>AQCSVDIQGNDQMQFNTNAITVDKSCKQFTVNLSHPGNLPKNVMGHDWVLSTAADMQGV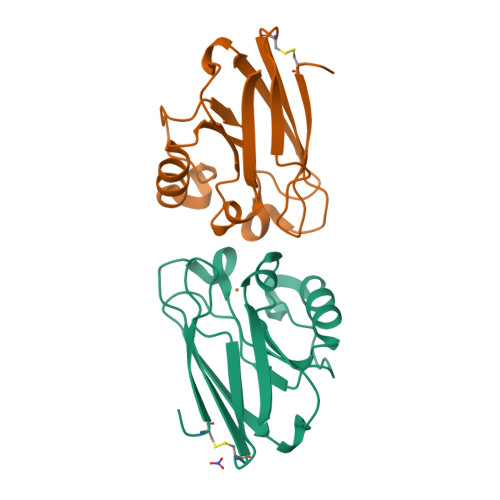VTDGMASGLDKDYLKPDDSRVIAHTKLIGSGEKDSVTFDVSKLKEGEQYMFFCTFPGHSALMKGTLTLK[4x]>[2x]MFSRPGLPVEYLQVPSASMGRDIKVQFQGGGPHAVYLLDGLRAQDDYNGWDINTPAFEEYYQSGLSVIMPVGGQSSFYTDWYQPSQSNGQNYTYKWETFLTREMPAWLQANKGVSPTGNAAVGLSMSGGSALILAAYYPQQFPYAASLSGFLNPSEGWWPTLIGLAMN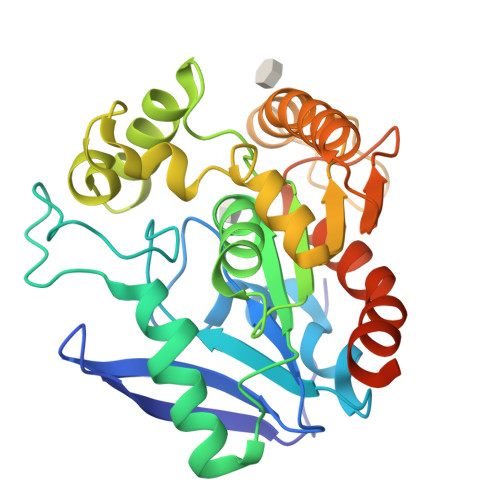DSGGYNANSMWGPSSDPAWKRNDPMVQIPRLVANNTRIWVYCGNGTPSDLGGDNIPAKFLEGLTLRTNQTFRDTYAADGGRNGVFNFPPNGTHSWPYWNEQLVAMKADIQHVLNGATPPAAPAAPAALGHHHHHH>LDPVFLAFAKLYIRDILDMKESRQVPGVFLYNGHPIKQVDVLGTVIGVRERDAFYSYGVDDSTGVINCICWKKLNTESVSAAPSAARELSLTSQLKKLQETIEQKTKIEIGDTIRVRGSIRTYREEREIHATTYYKVDDPVWNIQIARMLE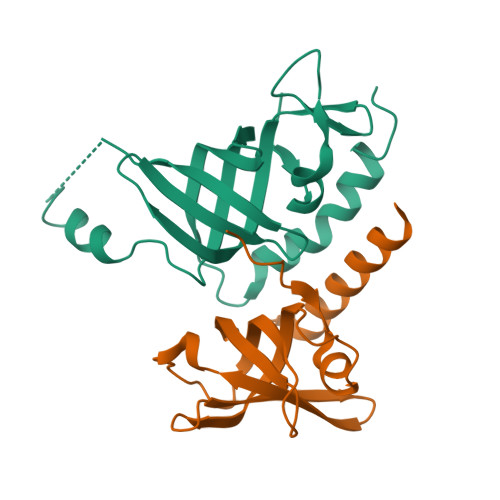LPTIYRKVYDQPFHS[2x];>[2x]MLPKPGTYYLPWEVSAGQVPDGSTLRTFGRLCLYDMIQSRVTLMAQHGSDQHQVLVCTKLVEPFHAQVGSLYIVLGELQHQQDRGSVVKARVLTCVEGMNLPLLEQAIREQRLYKQERGGSQ>[2x]MPLLLLLPLLWAGALAELHHHHHHENLYFQSGRYKCGISKACPEKHFAFKMASGAANVVGPKICLEDNVLMSGVKNNVGRGINIALVNGKTGEVIDTKFFDMWGGDVAPFIEFLKTIQDGTV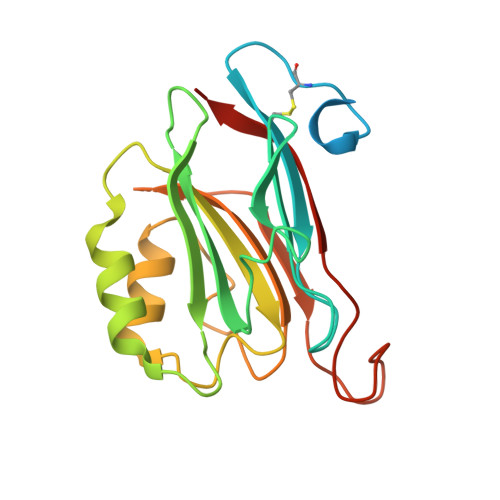VLMATYDDGATKLTDEARRLIAELGSTSITSLGFRDNWVFCGGKGIKTKSPFEQHIKNNKETNKYEGWPEVVEMEGCIPQKQD> MGDIMLIILTGLPG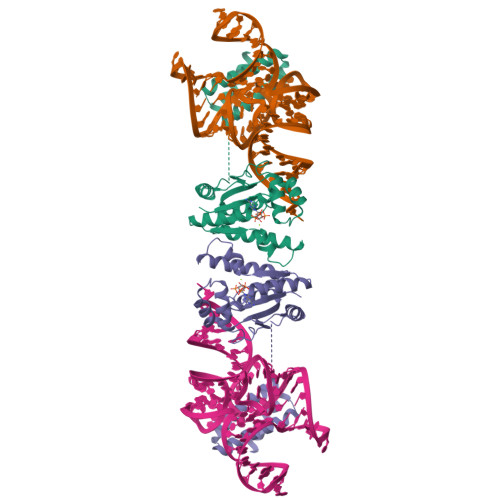VGKSTFSKNLAKILSKNNIDVIVLGSDLIRESFPVWKEKYEEFIKKSTYRLIDSALKNYWVIVDDTNYYNSMRRDLINIAKKYNKNYAIIYLKASLDVLIRRNIERGEKIPNEVIKKMYEKFDEPGKKYKWDEPFLIIDTTKDIDFNEIAKKLIEKSKEIPKFYVLEENKNKNNNISDKIDKETRKIVSEYIKSKKLDKDKIKEVVELRKEFLKKIKKMEEVDADRVLKEFKDLLNSYLEHHHHHH>MSTPRTTATAAKPKPYSFVNDYSVGMHPKILDLMARDNMTQHAGYGQDSHCAKAARLIGELLERPDADVHFISGGTQTNLIACSLALRPWEAVIATQLGHISTHETGAIEATGHKVVTAPCPDGKLRVADIESALHENRSEHMVIPKLVYISNTT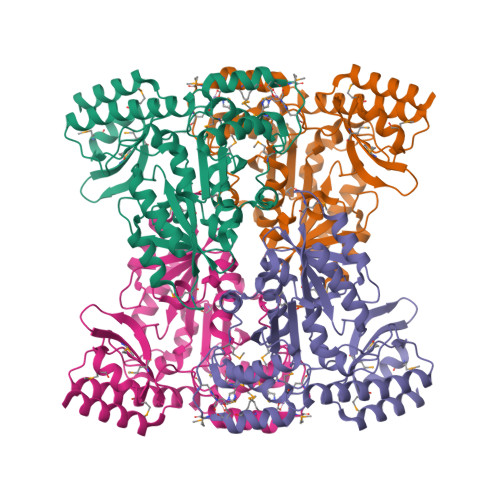EVGTQYTKQELEDISASCKEHGLYLFLDGARLASALSSPVNDLTLADIARLTDMFYIGATKAGGMFGEALIILNDALKPNARHLIKQRGALMAKGWLLGIQFEVLMKDNLFFELGAHSNKMAAILKAGLEACGIRLAWPSASNQLFPILENTMIAELNNDFDMYTVEPLKDGTCIMRLCTSWATEEKECHRFVEVLKRLVASTA[2x]> ATSWLLDGHLRAYTDDLARRLRGEPN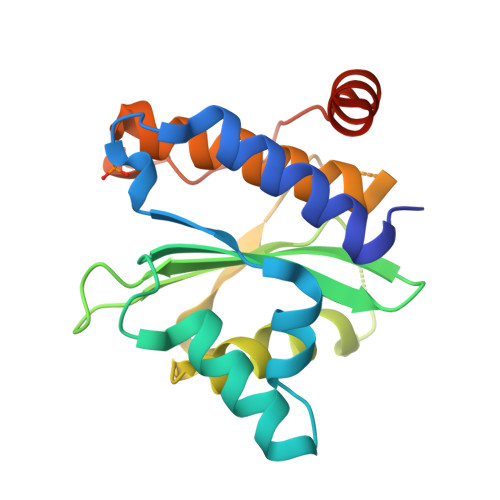AHLLHFADSQVVTMLSSADPDQQARAQRLLAGDDIPPIVFLPINQPNAHWSLLVVDRRNKDAVAAYHYDSMAQKDPQQRYLADMAAYHLGLDYQQTHEMPIAIQSDGYSCGDHVLTGIEVLAHRVLDGTFDYAGGRDLTDIEPDRGLIRDRLAQAEQAPA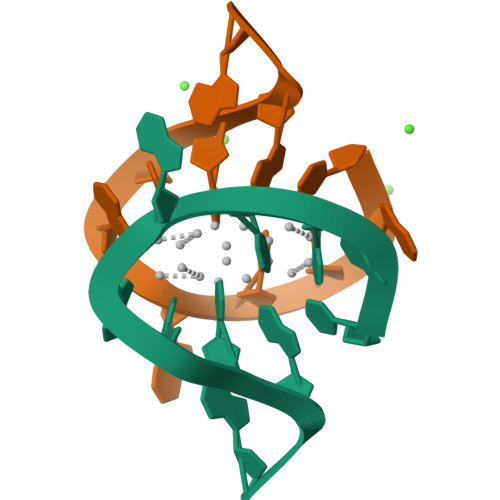>[4x]CACCAAGCGA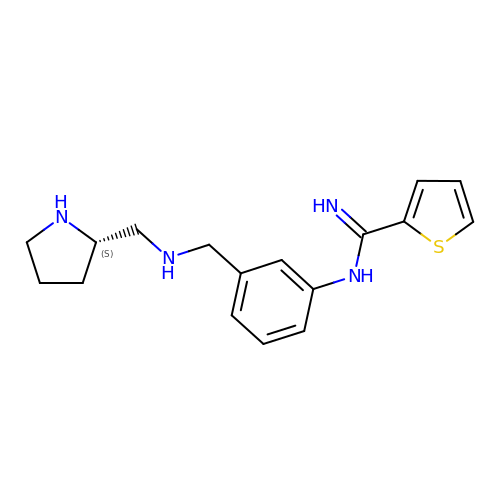(S)-N-(3-(((Pyrrolidin-2-ylmethyl)amino)methyl)phenyl)thiophene-2-carboximidamide | C17 H22 N4 S | MRTCFHYZEYSLIF-HNNXBMFYSA-N In recent years, the emergence of imine reductases (IREDs) has had a substantial impact on the application of enzymes in the preparation of chiral amines of pharmaceutical interest. IREDs are NAD(P)H-dependent oxidoreductases that catalyze the asymmetric reduction of prochiral imines, but in certain cases also enable the reductive amination of prochiral ketones through catalysis of both imine formation and subsequent reduction of the iminium ion intermediate. The enzyme designated IR77 by France and co-workers in a previous work has 100% sequence identity with NCBI accession sequence WP_053252429, annotated as an “NADP-binding domain” from the nitrogen-fixing bacterium Ensifer adhaerens, also known as a species of Sinorhizobium. The enzyme adopts the canonical fold now well established for IRED structures. An N-terminal Rossmann domain (residues 1–164) connects to a C-terminal helical domain (195–294) through a long alpha-helix (165–194). Two monomers closely associate in a domain swapping arrangement that serves to form two active sites per dimer, each at the interface of one N-terminal domain with the C-terminal domain of its partner.

Crystals were obtained in the P21 space group and featured four molecules, representing two dimers, in the asymmetric unit. In IR77, each dimer can be considered to be a “closed” structure, with a hydrophobic pocket formed at the cofactor binding site. The substrate binding site is defined by the frequently observed aspartate residue D171, which protrudes from the roof of the cavity into the active site from the interdomain helix. Facing the nicotinamide ring of the cofactor, on the opposite side of the active site, are the side chains of M178, W179, and H242 from the partner monomer. At the back of the active site are V212 and L216 from the partner monomer and T123. Two features of the active site which could explain the activity of the wild-type IR77 with bulkier imines are the presence of T209 and P241 at the back and front of the binding site as viewed in Figure 4B, which replace much larger tryptophan and methionine residues in IREDs that lack the ability to react with bulkier substrates, such as AspRedAm,7 and wild-type IR-G36.12. The product 2-cyclohexylisoindoline 1h was modeled into the active site of IR77 using Autodock Vina. Superimposition of the model with structures of AspRedAm clearly showed clashes with W210 and M239 in that enzyme with the cyclohexyl and aromatic rings of the substrate. The results suggest that the mode of catalysis of IR77 is therefore dependent on the nature of the amine partner in the reductive amination reaction, including size and its nucleophilicity in water, which may have a significant influence on the amount of imine formed in solution.

>[4x]MKPSISVLGTGRMGSALARALLQAGYRTVVWNRTSEKAEPLAALGATVAPTVRQAIDASGIVIVNVSDYAATSTLLRASDVTPGLRGKLIVELTSGTPEGARETSQWTAAHGARYLDGAILATPDFIGTDAGTILLSGALEPFAANEDVFRALGGNVQHIGTEPGLANALDSAVLALMWGALFGGLHAIAVCRAEEIDLGELGRQWAATAPVVEGLVADLIKRTSAGRFVSDAETLSSISPHYGAFQHLKELMEARRIDRTVVDGYDAIFRRAIASGHLHDDFAALSQFMGKAEQP>GHMAIAPNTRVLVAGYGLPAEFCVTTLIGMGVEIDKIAVATHREDNRNCGLHSMLRLRNIQFTTAAANSEEFYEFGANFAPDMIISMHYRSLIPGRFLKLAKKGSVNLHPSLLPAYRGTNSVAWVIINGESETGFSYHRMDENFDTGAILLQERIS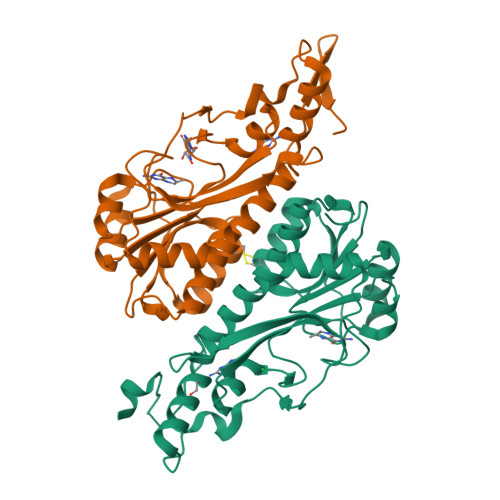VEETDTAFSLFHRQIARAMLRLEEVILKLDQGDPGFAQLGEASYYARELPFGGVIDPRWSEVQIDRFIRAMFFPPFPPAVLKIDGKVYYVPSIDIYRSLMRGIPS[2x]> MGSSHHHHHHSQDLMVTSTYIPMSQRRSWADVKPIMQDDGPNPVVPIMYSEEYKDAMDYFRAIAAKEEKSERALELTEIIVRMNPAHYTVWQYRFSLLTSLNKSLEDELRLMNEFAVQNLKSYQVWHHRLLLLDRISPQDPVSEIEYIHGSLLPDPKNYHTWAYLHWLYSHFSTLGRISEAQWGSELDWCNEMLRVDGRNNSAWGWRWYLRVSRPGAETSSRSLQDELIYILKSIHLIPHNVSAWNYLRGFLKHFSLPLVPILPAILPYTASKLNPDIETVEAFGFPMPSDPLPEDTPLPVPLALEYLADSFIEQNRVDDAAKVFEKLSSEYDQMRAGYWEFRRRECAE;> MATEFTPSVYSLVSKPLPSNSRPSATLDEQAETEDLISQLFDLTADPNALVSEHGKRYSGLRKQEHTQFLASSFFQLP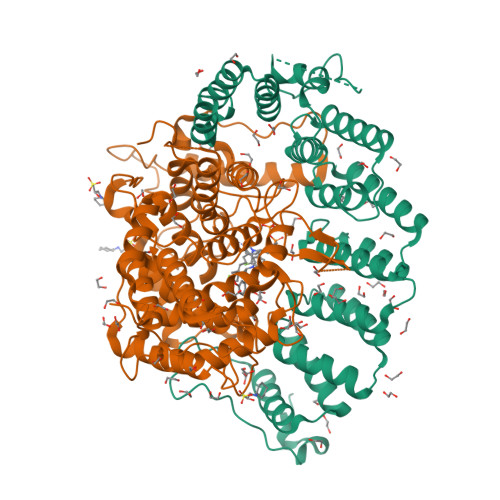GKFVSLDASRPWLVFWTVHSLDLLGVALDQGTKDRVVSTLLHFLSPKGGFGGGPANSQIPHLLPTYASVCSLAIAGNDSSTGGWKDLAAARQSIYEFFMRCKRPDGGFVVCEGGEVDVRGTYCLLVVATLLDIITPELLHNVDKFVSACQTYEGGFACASFPFPSVVPSTSAFPTSEPSCRVSMAEAHGGYTSCSLNSHFLLTSVPLPSFPLSIDANAALRWTVLQQGEPIEGGGFRGRTNKLVDGCYSWWVGGGAPVAEELVRREKSRKVKKSRIEVFEEEKEGDWEDVPPIPPIFNRVALQEFTLVAAQQDPGSTGGLRDKPGKRPDQYHTCNNLSGLSIAQHKMSHSPSTVSSNRLKFDASKGLPAVKPVAPGGGWKNEDERQNARREIWANALGWIEEEGGEIIVGGKDNRINTTTPVFNILGLRLKPFINYFYCQEN> MGNKSDAAAKQIKKLEEDFDGRIGVFAIDTGSGNTFGYRSDERFPLCSSFKGFLAAAVLERVQQKKLDINQKVKYESRDLEYHSPITTKYKGSGMTLGDMASAALQYSDNGATNIIMERFLGGPEGMTKFMRSIGDNEFRLDRWELELNTAIPGDKRDTSTP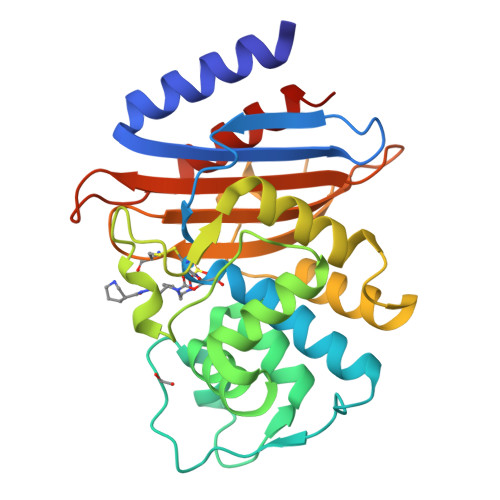KAVANSLNKLALGNVLNAKVKAIYQNWLKGNTTGDARIRASVPADWVVGDKTGSCGAYGTANDYAVIWPKNRAPLIVSIYTTRKSKDDKHSDKTIAEASRIAIQAIDHHHHHH> LADQQDLTRQVPAEVESLDPAHIESWTGNTIGLDLFEGLARIDASGAVVPGVAQAWEHKAPDTWIFKLRRDAKWSNGQPVTAADFVYAWQRLADPKTGSKYTILVEFVKNASAIIAGKQPPGDLGIRAIDPYTIEVKTEVPVSYFPELTAMAPLTPVNKDAVAKFGDAWTRPKNIVSNGPYTLVDWQPNNRIVMAKSDKYWNARNVVIRKVTYLPIENDETALRMYQAGQIDYTYSIPAGGFGQISKQFGKELRPGLQLATYYYYLKNSDPALKDKRVREALAMVLDREILTSKITQAGEVPMYGLMPK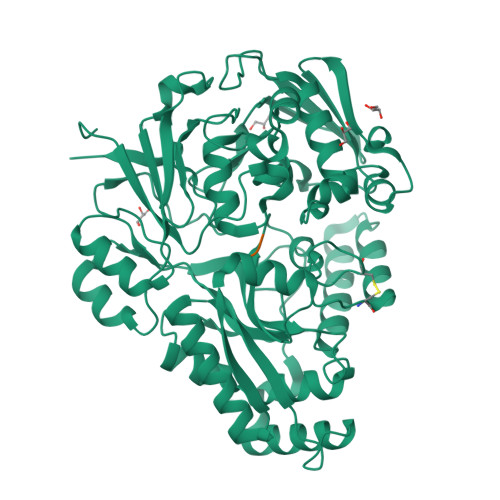GVKGVQRPFTPDWASWPMARRVDYAKNLLKQAGHGDANPLTFTLTYNTNDLHKKVALFAASEWRTKLGVTAKLENVEFKVLMKQRHDGKVQIARDGWFADYNDAMTFFDLIRCGSSQNTVGYCNPKVDSLVAEANQKLDDGARAALLTQAHDLAMNDYPMVPLFQYSADRLVKSYVGGYTLTNYIDMRASQDMYLIK;> DVA> MGKSASKQFHNEVLKAHNEYRQKHGVPPLKLCKNLNREAQQYSEALASTRILKHSPESSRGQCGENLAWASYDQTGKEVADRWYSEIKNYNFQQPGFTSGTGHFTAMVWKNTKKM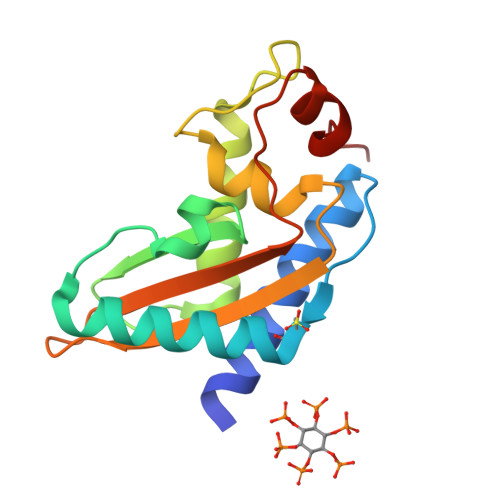GVGKASASDGSSFVVARYFPAGNVVNEGFFEENVLPPKK> KEDFVGHQVLRITAADEAEVQTVKELEDLEHLQLDFWRGPGQ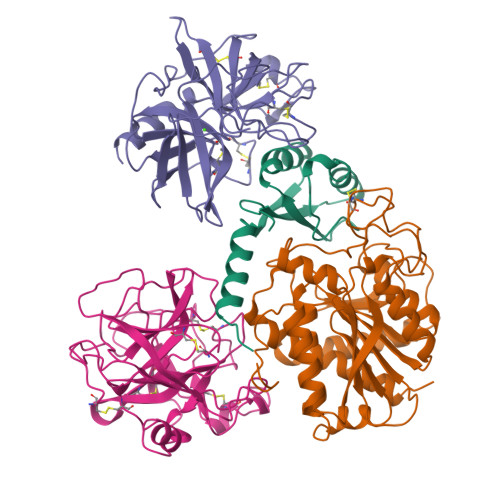PGSPIDVRVPFPSLQAVKVFLEAHGIRYRIMIEDVQSLLDEEQEQMFASQSR;> ARSTNTFNYATYHTLDEIYDFMDLLVAEHPQLVSKLQIGRSYEGRPIYVLKFSTGGSNRPAIWIDLGIHSREWITQATGVWFAKKFTEDYGQDPSFTAILDSMDIFLEIVTNPDGFAFTHSQNRLWRKTRSVTSSSLCVGVDANRNWDAGFGKAGASSSPCSETYHGKYANSEVEVKSIVDFVKDHGNFKAFLSIHSYSQLLLYPYGYTTQSIPDKTELNQVAKSAVEALKSLYGTSYKYGSIITTIYQASGGSIDWSYNQGIKYSFTFELRDTGRYGFLLPASQIIPTAQETWLGVLTIMEHTLNNLY;> FSQPFSRPSSRVVNGEDAVPYSWSWQVSLQYEKDGAFHHTCGGSLIAPDWVVTAGHCISTSRTYQVVLGEYDRSVLQGSEQVIPINAGDLFVHPLWNSNCVACGNDIALVKLSRSAQLGDKVQLANLPPAGDILPNEAPCYISGWGRLYTGGPLPDKLQEALLPVVDYEHCSQYDWWGITVKKTMVCAGGDTRSGCDGDSGGPLNCPAADGSWQVHGVTSFVSAFGCNTIKKPTVFTRVSAFIDWINETIASN;> CGAPIFQPNLSARVVGGEDAIPHSWPWQISLQYLRDNTWRHTCGGTLITPNHVLTAAHCISNTLTYRVALGKNNLEVEDEAGSLYVGVDTIFVHEKWNSFLVRNDIALIKLAETVELGDTIQVACLPSEGSLLPQDYPCFVTGWGRLYTNGPIAAELQQGLQPVVDYATCSQRDWWGTTVKETMVCAGGDGVISACNGDSGGPLNCQADGQWDVRGIVSFGSGLSCNTFKKPTVFTRVSAYIDWINQKLQL>[2x]MAKNHYDILRRHIRSEDLLETPEFGSGSRIVEEYWIQEPFTKAIIVENEDEFRNVYYALEPTVSSEEAEVISALYDDLKKILVLQDVSVDLEERAEVLVRAIEKLSKEYAVSFTDNFYSRMLYYLFRDFFGYGLIDPLMEDTNVEDISCDGYNIPIFIYHQKYGNVETNIVLDQEKLDRMVLRLTQRSGKHISIANPIVDATLPDGSRLQATFGTEVTPRGSSFTIRKFTIEPLTPIDLIEKGTVPSGVLAYLWLAIEHKFSAIVVGETASGKTTTLNAIMMFIPPDAKVVSIEDTREIKLYHENWIAEVTRTGMGEGEIDMYDLLRAALRQRPDYIIVGEVRGREAQTLFQAMSTGHASYSTLHAGDINQMVYRLESEPLKVPRSMLQFLDIALVQTMW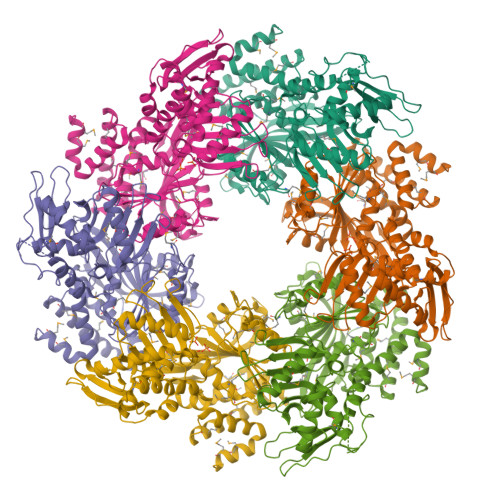VRGNTRLRRTKEVNEILGIDPVDKNLLVNQFVKWDPKEDKHIEVSMPKKLEKMADFLGVSVQEVYDEMLSRKRYLELMLKRGIRNYKEVTRYIHAYYRNPELAMTKMEEGL>[2x]GHMSLEEWIKADSLEKADEYHKRYNYAVTNPVRRKILRMLDKGRSEEEIMQTLSL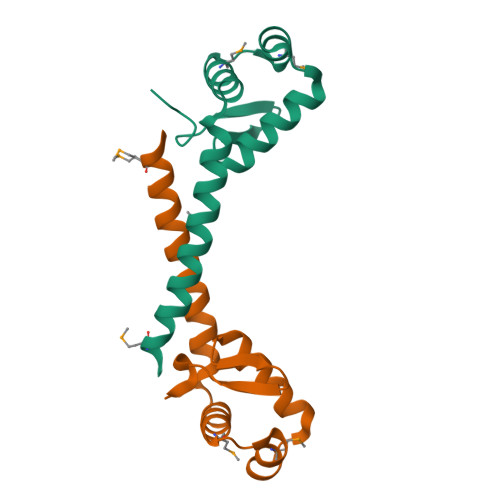SKKQLDYHLKVLEAGFCIERVGERWVVTDAGKIVDKIRGGS> MSLTREAYHRLTPLPHPGGRLFIKPGARGYRDPVHDLLQKTVEPFGERALDLNPGVGWGSLPLEGRMAVERLETSRAAFRCLTASGLQARLALPWEAAAGAYDLVVLALPAGRGTAYVQASLVAAARALRMGGRLYLAGDKNKGFERYFKEARALLGYGVVVRREGPYRVALLEKEKEAPPLPSLWRAFSARILGAEYTFHHLPGVFSAGKVDPASLLLLEALQERLGPEGVRGRQVLDLGAGYGALTLPLARMGAEVVGVEDDLASVLSLQKGLEANALKAQALHSDVDEALTEEARF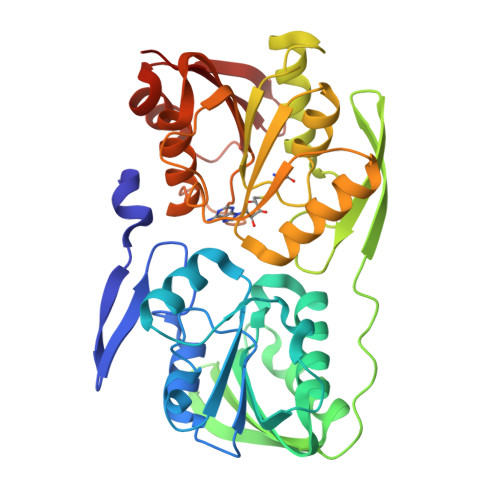DIIVTNPPFHVGGAVILDVAQAFVNVAAARLRPGGVFFLVSNPFLKYEPLLEEKFGAFQTLKVAEYKVLFAEKRGR>[2x]MKPYQRQFIEFALSKQVLKFGEFTLKSGRKSPYFFNAGLFNTGRDLALLGRFYAEALVDSGIEFDLLFGPAY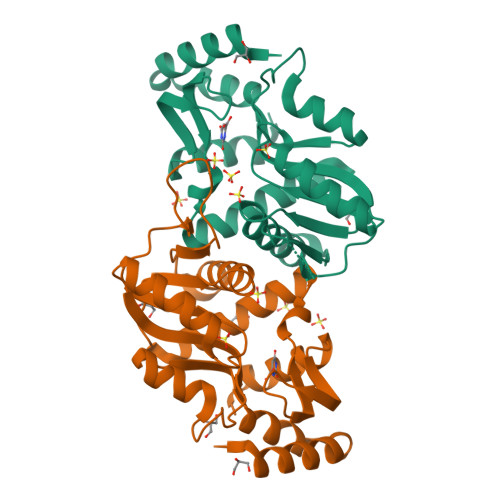KGIPIATTTAVALAEHHDLDLPYCFNRKEAKDHGEGGNLVGSALQGRVMLVDDVITAGTAIRESMEIIQANGATLAGVLISLDRQERGRGEISAIQEVERDYNCKVISIITLKDLIAYLEEKPEMAEHLAAVKAYREEFGV>[4x]MAASELYTKYARVWIPDPEEVWKSAELLKDYKPGDKVLQLRLEEGKDLEYCLDPKTKELPPLRNPDILVGENDLTALSYLHEPAVLHNLKVRFIDSKLIYTYCGIVLVAINPYEQLPIYGEDIINAYSGQNMGDMDPHIFAVAEEAYKQMARDERNQSIIVSGESGAGK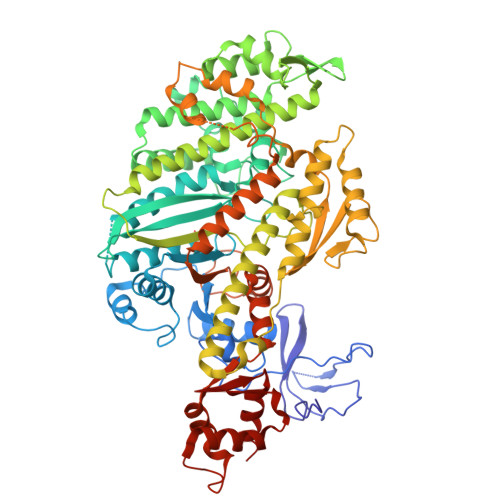TVSAKYAMRYFATVSGSASEANVEEKVLASNPIMESIGNAKTTRNDNSSRFGKYIEIGFDKRYRIIGANMRTYLLEKSRVVFQAEEERNYHIFYQLCASAALPEFKTLRLGNANYFHYTKQGGSPVIDGIDDAKEMVNTRQACTLLGISDSYQMGIFRILAGILHLGNVEFASRDSDSCAIPPKHDPLTIFCDLMGVDYEEMAHWLCHRKLATATETYIKPISKLHAINARDALAKHIYANLFNWIVDHVNKALHSTVKQHSFIGVLDIYGFETFEINSFEQFCINYANEKLQQQFNMHVFKLEQEEYMKEQIPWTLIDFYDNQPCINLIEAKMGVLDLLDEECKMPKGSDDTWAQKLYNTHLNKCALFEKPRLSNKAFIIKHFADKVEYQCEGFLEKNKDTVYEEQIKVLKSSKKFKLLPELFQDEEKAISPTSATPSGRVPLSRTPVKPAKARPGQTSKEHKKTVGHQFRNSLHLLMETLNATTPHYVRCIKPNDFKFPFTFDEKRAVQQLRACGVLETIRISAAGFPSRWTYQEFFSRYRVLMKQKDVLSDRKQTCKNVLEKLILDKDKYQFGKTKIFFRAGQVAYLEKIRADK>SARVGSQNGVQMLSPSEIPQRDWFPSDFTFGAATSAYQIEGAWNEDGKGESNWDHFCHNHPERILDGSNSDIGANSYHMYKTDVRLLKEMGMDAYRFSISWPRILPKGTKEGGINPDGIKYYRNLINLLLENGIEPYVTIFHWDVP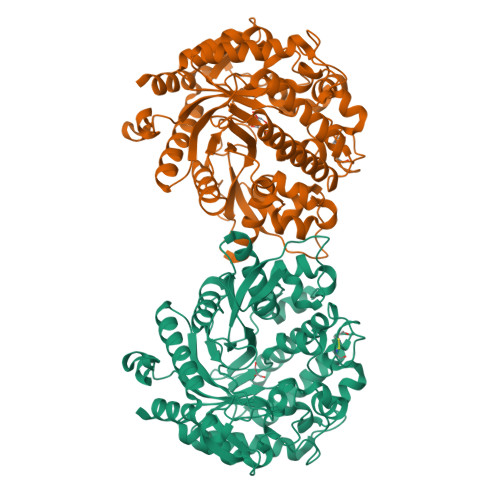QALEEKYGGFLDKSHKSIVEDYTYFAKVCFDNFGDKVKNWLTFNDPQTFTSFSYGTGVFAPGRCSPGLDCAYPTGNSLVEPYTAGHNILLAHAEAVDLYNKHYKRDDTRIGLAFDVMGRVPYGTSFLDKQAEERSWDINLGWFLEPVVRGDYPFSMRSLARERLPFFKDEQKEKLAGSYNMLGLNYYTSRFSKNIDISPNYSPVLNTDDAYASQEVNGPDGKPIGPPMGNPWIYMYPEGLKDLLMIMKNKYGNPPIYITENGIGDVDTKETPLPMEAALNDYKRLDYIQRHIATLKESIDLGSNVQGYFAWSLLDNFEWFAGFTERYGIVYVDRNNNCTRYMKESAKWLKEFNTAKKPSKKILTPA[2x]>MKVQYCDSLVIGGGLAGLRAAVATQQKGLSTIVLSLIPVKRSHSAAAQGGMQASLGNSKMSDGDNEDLHFMDTVKGSDWGCDQKVARMFVNTAPKAIRELAAWGVPWTRIHKGDRMAIINAQKTTITEEDFRHGLIHSRDFGGTKKWRTCYTADATGHTMLFAVANECLKLGVSIQDRKEAIALIHQDGKCYGAVVRDLVTGDIIAYVAKGTLIATGGYGRIYKNTTNAVVCEGTGTAIALETGIAQLGNMEAVQFHPTPLFPSGILLTEGCRGDGGILRDVDGHRFMPDYEPEKKELASRDVVSRRMIEHIRKGKGVQSPYGQHLWLDISILGRKHIETNLRDVQEICEYFAGIDPAEKWAPVLPMQHYSMGGIRTDYRGEAKLKGLFSAGEAACWDMHGFNRLGGNSVSEAVVAGMIVGEYFAEHCANTQVDLETKTLEKFVKGQEAYMKSLVESKGTEDVFKIKNRMKDVMDDNVGIFRDGPHLEKAVKELEELYKKSKNVGIKNKRLHANPELEEAYRVPMMLKVALCVAKGALDRTESRGAHNREDYPKRDDINWLNRTLASWPNPEQTLPTLEYEALDVNEMEIAPGYRGYGAKGNYIENPLSVKRQEEIDKIQSELEAAGKDRHAIQEALMPYELPAKYKARNERLGDK[2x];>[2x]MGRMLTIRVFKYDPQSAVSKPHFQEYKIEEAPSMTIFIVLNMIRETYDPDLNFDFVCRAGI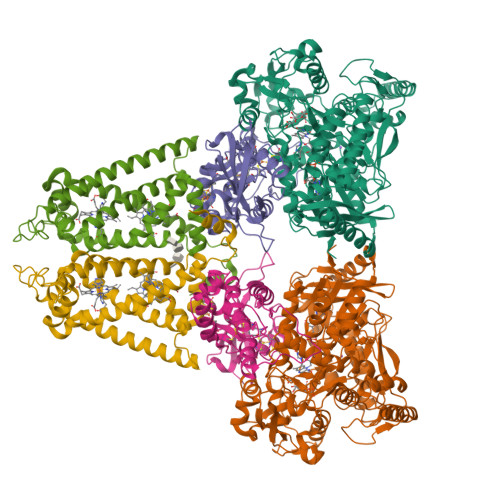CGSCGMMINGRPSLACRTLTKDFEDGVITLLPLPAFKLIKDLSVDTGNWFNGMSQRVESWIHAQKEHDISKLEERIEPEVAQEVFELDRCIECGCCIAACGTKIMREDFVGAAGLNRVVRFMIDPHDERTDEDYYELIGDDDGVFGCMTLLACHDVCPKNLPLQSKIAYLRRKMVSVN;>[2x]MTNESILESYSGVTPERKKSRMPAKLDWWQSATGLFLGLFMIGHMFFVSTILLGDNVMLWVTKKFELDFIFEGGKPIVVSFLAAFVFAVFIAHAFLAMRKFPINYRQYLTFKTHKDLMRHGDTTLWWIQAMTGFAMFFLGSVHLYIMMTQPQTIGPVSSSFRMVSEWMWPLYLVLLFAVQLHGSVGLYRLAVKWGWFDGETPDKTRANLKKLKTLMSAFLIVLGLLTFGAYVKKGLEQTDPNIDYKYFDYKRTHHR> MGSDKIHHHHHHENLYFQGMSFKNFKCVPKMIFGRGSFVQLDTVLEQERTDANDFVVFLVDDVHQHKPLAARVPNKAHDLVIYVNVDDEPTTVQVDELTAQVKAFNTKLPVSVVGLGGGSTMDLAKAVSLMLTNPGSSSEYQGWDLIKNPAVHHIGIPTVSGTGAEASRTAVLCGPVRKLGLNSDYTVFDQIIMDSELIAGVPTDQWFYTGMDCFIHCVESLQGTYLNEFAKAFAEKSMDLCREVYLDDHPEKDDKLMMASYMGGMSIAYSQVGACHAVSYGLGYVLGYHHGIGNCLAFDVLE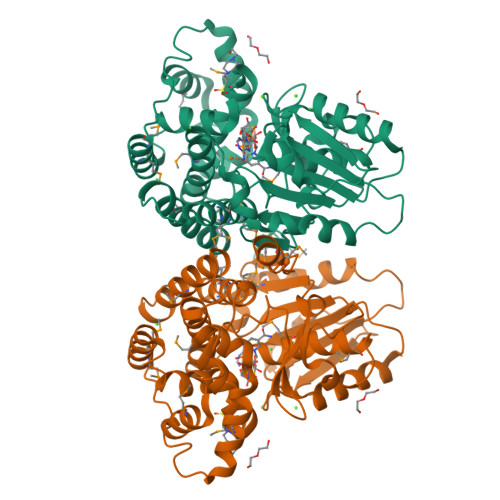EFYPEGVAEFRKMMEIHNITLPKNICKDLPDETIAKMVAVTKSMGPLWDNVYGKGWEEKVTDEMLTKLFRRI3-(benzoylamino)-N-oxobenzamide | C14 H10 N2 O3 | 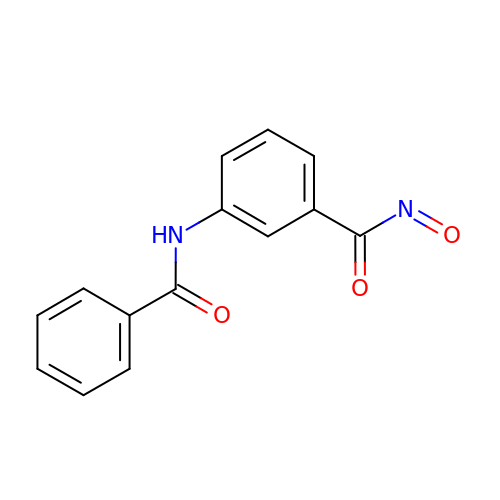BZGLPPUMZXGKFN-UHFFFAOYSA-N> MIVGVGIDVLEVERVPEKFAERILGESEKRLFLTRKRRREFIAGRFALKEAFFKALGTGLNGHSFTDVEFLESNGKPVLCVHKDFGFFNYAHVSLSHDRFAVALVVLEKRK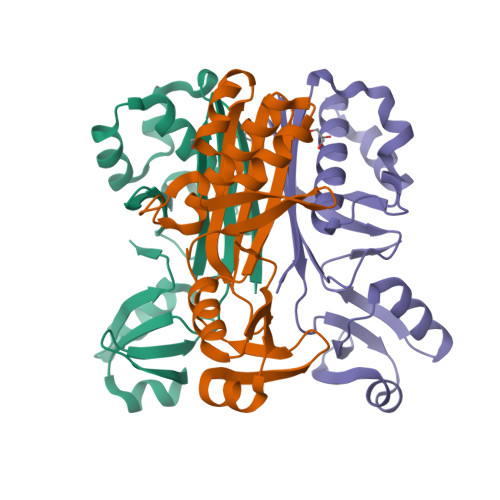GDIIVEGDESFLRKRFEVLERSVEGWEIETSLPPFTLKKLLESSGCRLVRYGNILIGE>[7x]GPHMVRKQEIIKVNQQLIEAISNGDFESYTKMCDPGMTAFEPEALGNLVEGLDFHRFYFENLWSRNSKPVHNTMLNPHIHLMGDESA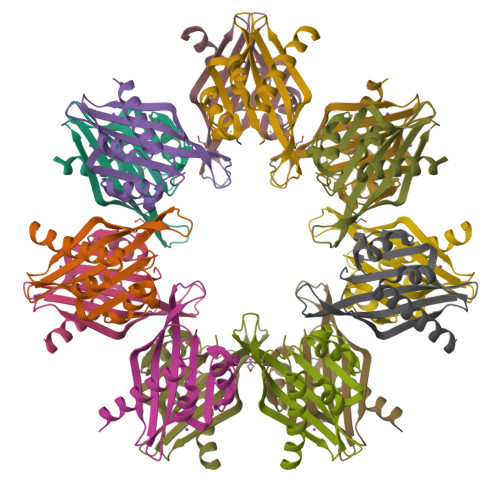CIAYIRITQYLDAGGIPRTAQSEETRVWHRRDGKWQHVHMHRSGAPSV>MPLPKTHELHIFGSFNGVKFDMVGEGTGNPNEGSEELKLKSTNGPLKFSPYILVPHLG[2x];>[2x]YAFNQYLPFPDGMSPFQAAMQDESGYQVHRTLQYEDGAFVTANLRYTYEGSHIKGEFQVIGTGFPPDGPVMTNKLTALDWSVVKFVYPNDKTILSTFD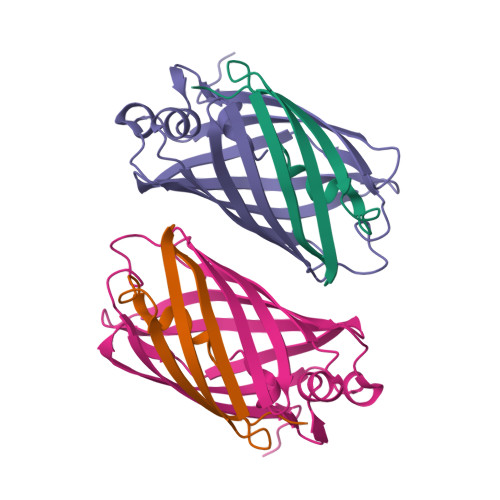KTYTTTDGKRYQCTFRENNTFAKPMAADILQKQPMFIFHKTELQHSNNAELTFKEKQTAFSDMKSGGSHHHHHH1-[4-({(1R)-1-[(6S,7S)-2-amino-7-methyl-4-oxo-1,4,5,6,7,8-hexahydropteridin-6-yl]ethyl}amino)phenyl]-1-deoxy-5-O-{5-O-[(R)-{[(1R)-1,3-dicarboxypropyl]oxy}(hydroxy)phosphoryl]-alpha-D-ribofuranosyl}-D-xylitol 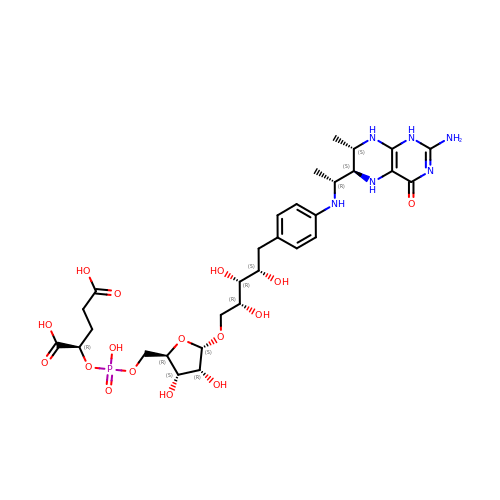| C30 H45 N6 O16 P | SCBIBGUJSMHIAI-FQVOATFZSA-N>[2x]ASSNANQAITSENSIKPKGKLQPQMEKYTLTYFNGRGRAEVIRLLFALANVSYEDNRITRDEWKYLKPRTPFGHV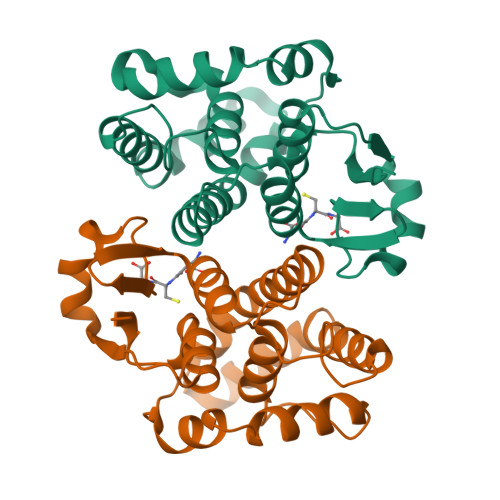PMLNVSGNVLGESHAIELLLGGRFGLLGTNDWEEAKIMAVVLNIDELFQKLIPWTHEKNTTKKAELFRNLSESDVMPFLGRYEKFLKESTTGHIVGNKVSVADLTVFNMLMTLDDEVKLEEYPQLASFVNKIGQMPGIKEWIKKRPKTYF As evidenced by the fact that their genetic ablation led to compromised K+ permeability and Ca2+ release across the SR/ER membrane, TRICs play important roles as counter-ion channels for balancing the charge potential change during Ca2+ release/uptake in the intracellular stores. In this study, we analyse the structure and function of a bacterial and an archaeal TRIC channel. Both proteins have similar structures, consisting in symmetric trimers of 7-TM subunits, each composed as inverted quasi-repeats of triple-helix bundles (THBs) plus an added TM segment (TM7). Many other trimeric channels, including ATP-gated P2X receptors, acid-sensing ion channels40 and the mechanosensitive Piezo1 channels41, form central ion-conducting pores at the three-fold axes of protomer association; by contrast, the prokaryotic TRIC trimers have three pores as calculated by the HOLE programme, one through each protomer.

Different from SaTRIC, the bacterial CpTRIC was solubilized in octylmaltoside (OM) and crystallized from detergent micelles in space group R32, with one protomer per ASU. This structure was solved to 2.4 Å resolution by Se-SAD. The final model for CpTRIC was refined to Rwork/Rfree values of 24.0%/27.5%, containing ordered residues 3–198, 5 Cd2+ ions and 27 water molecules. Overall, the two prokaryotic TRICs are very similar, with a root mean squared deviation (r.m.s.d.) of 1.39 Å when 188 Cα atoms are superimposed. Interestingly, each homologous repeat forms a structurally similar THB, with r.m.s.d. of 1.32 Å/79 Cα for SaTRIC and r.m.s.d. of 1.45 Å/71 Cα for CpTRIC. Another ion-binding site was also observed at an inter-protomer interface in the trimeric channel of CpTRIC. One Cd2+ ion was bound to a well-conserved Asp residues (D40 in CpTRIC, located at the N-terminal end of the GGG-kinked TM2), and interacting with several backbone carbonyl oxygen or nitrogen from the short linker between TM5′ and TM6′ on the adjacent protomer (residues 145–149 in CpTRIC). In keeping with the closer similarity of SsTRIC to the closed conformation of SaTRIC, an H-bonded network of interactions closes the C-THB in a locked conformation in both SsTRIC and RsTRIC, just as in the structures of both SaTRIC type 2b and CpTRIC.

> MNDFLFYLDIFGVIVFALSGALMAGRYQLDPFGVVVLASVTAVGGGTIRDVILQTPVFWVEKPYYLYVILATAILTIVLIRQPKRIPKRFLLIADALGLALFAVLGTQKALYLGAPIPVAVVLGTITGIAGGMIRDVLCNVIPMILREEIYALAAMLGGSLFIILHGLNWNDTNAMIVSISAALALRLAAIYWHVSLPAFHIVEKPKKEKGTTKIIEKKAAAENLYFQGLEDYKDDDDKHHHHHHHHHH> AEAGITGTWYAQLGDTFIVTAGADGALTGTYEAAVGNAESRYVLTGRYDSA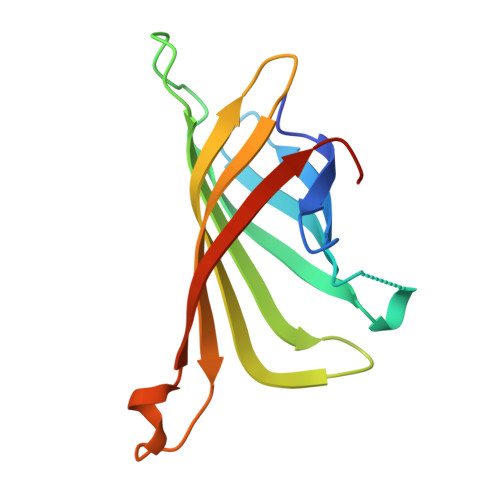PATDGSGTALGWTVAWKNNYRNAHSATTWSGQYVGGAEARINTQWLLTSGTTEANAWKSTLVGHDTFTKVKPSAAS> DPSNVETYEQILQWVTEVLGNDIPHDLIIGTADIFIRQLKENEENEDGNIEERKEKIQHELGINIDSLKFNELVKLMKNINKRALPNIENDIIKLSDSKTSNIESVPIYSIDEFFLQRKLRSELGYKDTSVIQDLSEKILNDIETLEHNPVALEQKLVDLLKFENISLAEFILKNRSTIFWGIRLAKSTENEIPNLIEKMVAKGLNDLVEQYKFRENPAIPPVIDLEKIKFDESSKLMTVTKVSLPEGSFKRVKPQYDEIHIPAPSKPVIDYELKEITSLPDWCQEAFPSSETTSLNPIQSKVFHAAFEGDSNMLICAPTGSGKTNIALLTVLKALSHHYNPKTKKLNLSAFKIVYIAPLKALVQEQVREFQRRLAFLGIKVAELTGDSRLSRKQIDETQVLVSTPEKWDITTRNSNNLAIVELVRLLIIDEIHLLHDDRGPVLESIVARTFWASKYGQEYPRIIGLSATLPNYEDVGRFLRVPKEGLFYFDSSFRPCPLSQQFCGIKERNSLKKLKAMNDACYEKVLESINEGNQIIVFVHSRKETSRTATWLKNKFAEENITHKLTKNDAGSKQILKTEAANVLDPSLRKLIESGIGTHHAGLTRSDRSLSEDLFADGLLQVLVCTATLAWGVNLPAHTVIIKGTDVYSPEKGSWEQLSPQDVLQMLGRAGRPRYDTFGEGIIITDQSNVQYYLSVLNQQLPIESQFVSKLVDNLNAEVVAGNIKCRNDAVNWLAYTYLYVRMLASPMLYKVPDISSDGQLKKFRESLVHSALCILKEQELVLYDAENDVIEATDLGNIASSFYINHASMDVYNRELDEHTTQIDLFRIFSMSEEFKYVSVRYEEKRELKQLLEKAPIPIREDIDDPLAKVNVLLQSYFSQLKFEGFALNSDIVFIHQNAGRLLRAMFEICLKRGWGHPTRMLLNLCKSATTKMWPTNCPLRQFKTCPVEVIKRLEASTVPWGDYLQLETPAEVGRAIRSEKYGKQVYDLLKRFPKMSVTCNAQPITRSVMRFNIEIIADWIWDMNVHGSLEPFLLMLEDTDGDSILYYDVLFITPDIVGHEFTLSFTYELKQHNQNNLPPNFFLTLISENWWHSEFEIPVSFNGFKLPKKFPPPTPLLENISISTSELGNDDFSEVFEFKTFNKIQSQVFESLYNSNDSVFVGSGKGTGKTAMAELALLNHWRQNKGRAVYINPSGEKIDFLLSDWNKRFSHLAGGKIINKLGNDPSLNLKLLAKSHVLLATPVQFELLSRRWRQRKNIQSLELMIYDDAHEISQGVYGAVYETLISRMIFIATQLEKKIRFVCLSNCLANARDFGEWAGMTKSNIYNFSPSERIEPLEINIQSFKDVEHISFNFSMLQMAFEASAAAAGNRNSSSVFLPSRKDCMEVASAFMKFSKAIEWDMLNVEEEQIVPYIEKLTDGHLRAPLKHGVGILYKGMASNDERIVKRLYEYGAVSVLLISKDCSAFACKTDEVIILGTNLYDGAEHKYMPYTINELLEMVGLASGNDSMAGKVLILTSHNMKAYYKKFLIEPLPTESYLQYIIHDTLNNEIANSIIQSKQ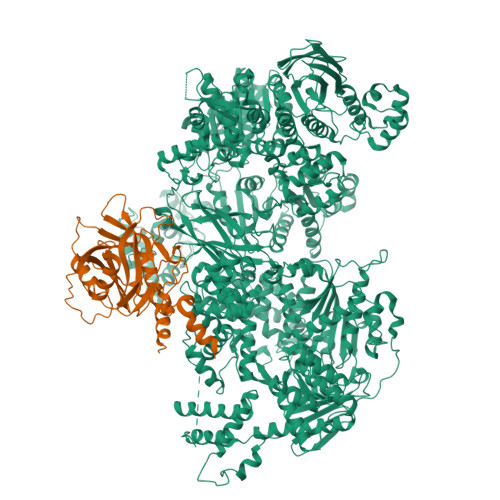DCVDWFTYSYFYRRIHVNPSYYGVRDTSPHGISVFLSNLVETCLNDLVESSFIEIDDTEAETEIISTLSNGLIASHYGVSFFTIQSFVSSLSNTSTLKNMLYVLSTAVEFESVPLRKGDRALLVKLSKRLPLRFPEHTSSGSVSFKVFLLLQAYFSRLELPVDFQNDLKDILEKVVPLINVVVDILSANGYLNATTAMDLAQMLIQGVWDVDNPLRQIPHFNNKILEKCKEINVETVYDIMALEDEERDEILTLTDSQLAQVAAFVNNYPNVELTYSLNNSDSLISGVKQKITIQLTRDVEPENLQVTSEKYPFDKLESWWLVLGEVSKKELYAIKKVTLNKETQQYELEFDTPTSGKHNLTIWCVCDSYLDADKELSFEINVK;> SKNEWRKSAIANTLLYLRLKNIYVSADDFVEEQNVYVLPKNLLKKFIEISDVKIQVAAFIYGMSAKDHPKVKEIKTVVLVPQLGHVGSVQISNIPDIGDLPDTEGLELLGWIHTQTEELKFMAASEVATHSKLFADKKRDCIDISIFSTPGSVSLSAYNLTDEGYQWGEENKDIMNVLSEGFEPTFSTHAQLLLSDRITGNFIIPSGNVWNYTFMGTAFNQEGDYNFKYGIPLEFYNEMHRPVHFLQFSEL> RILPEVK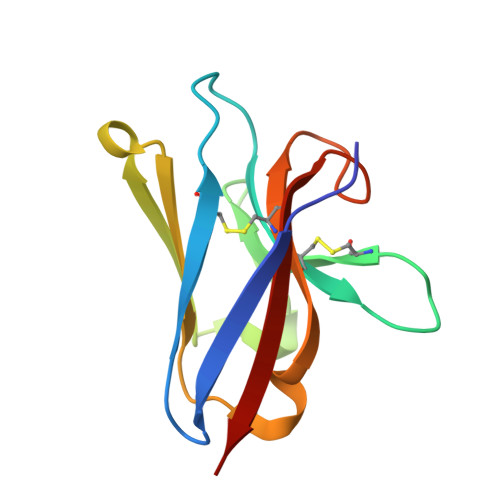VEGELGGSVTIKCPLPEMHVRIYLCREMAGSGTCGTVVSTTNFIKAEYKGRVTLKQYPRKNLFLVEVTQLTESDSGVYACGAGMNTDRGKTQKVTLNVHS> ATFLIWPIYPKIEANEKATAVWLQNTGKTDAMVQIRVFKWNQDGLKDNYSEQSEIIPSPPVAKIKAGEKHMLRLTKSVNLPDGKEQSYRLIVDELPIRLSDGNEQDASKVSFQMRYSIPLFAYGKGIGSGLTEESQKLNAKNALAKPVLQWSVRNNQQGQSELYLKNNGQKF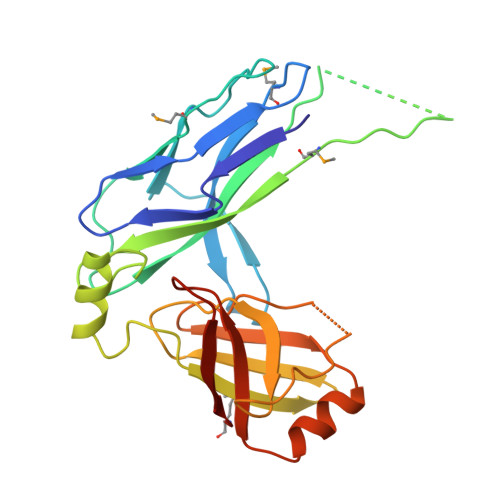ARLSALKTSKTGNDISLGKAAFGYVLSNSTVKFAIDQSTAHELAKTSKIYGVDSSGIKQELIEITKMEDPS> MAELRMEHIYKFYDQKEPAVDDFNLHIADKEFIVFVGPSGCGASTTLRMVAGLEEISKGDFYIEGKRVNDVAPKDRDIAMVFQNYALYPHMTVYDNIAFGLKLRKMPKPEIKKRVEEAAKILGLEEYLHRKPKALSGGQRQRVALGRAIVRDAKVFLMDEPLSNLDAKLRVQMRAEIIKLHQRLQTTTIYVTHDQTEALTMATRIVVMKDGKIQQIGTPKDVYEFPENVFVGGFIGSPAMNFFKGKLTDGLIKIGSAALTVPEGKMKVLREKGYIGKEVIFGIRPEDIHDELIVVESYKNSSIKAKINVAELLGSEIMIYSQIDNQDFIARIDARLDIQSGDELTVAFDMNKGHFFDSETEVRIRLEHHHHHH

ABC exporters and importers share a core structural design composed of at least two intracellular nucleotide-binding domains (NBDs) and two transmembrane domains (TMDs) embedded in the lipid bilayer that form the translocation pore, and the same mechanism of ATP binding and catalysis to energize the movement of substrates across the membrane. Later, our laboratory and others demonstrated that Gram-positive bacteria have orphan NBDs that are able to energize multiple ABC type I sugar importers. Finally, we solve the crystal structure of the B. subtilis multitask ATPase MsmX K43A; the crystals diffracted up to 1.67 Å resolution and based on comparative analysis we hypothesize about sequence and structural features involved in the broader specificity of NBDs. MsmX K43A shares the fold of well-studied NBDs of ABC type I importers.

K43 is involved in ATP coordination and catalysis, interacting with the β- and γ-phosphate groups. Its replacement by an alanine resulted in 80% decreased ATPase activity, impairing the normal function of MsmX to energize the AraNPQ transporter in B. subtilis. The crystal structure was solved at 1.67 Å resolution and the final electron density map allowed to model a detailed refined structure, which comprises all residues of MsmX K43A, except the N-terminus methionine. Interestingly, most crystal structures of NBDs from ABC transporters show a dimer in the asymmetric unit, promoted either by the C-terminal domains or the presence of ATP (or analogs). This is not the case for B. subtilis MsmX, that crystallized as a monomer with one molecule in the asymmetric unit, and very few contacts with symmetry related molecules, as indicated by analyzing the protein interface using PISA server. MsmX N-terminal domain presents the general α/β-type ATPase domain fold, which comprises the RecA-like domain (residues 2–87 and 155–235, in blue) and the α-helical domain (residues 88–154, in yellow). The regulatory C-terminal domain (residues 236–365, in red) forms a mixed barrel with 3 α-helices and 11 β-strands. In the ligand-free MsmX K43A structure here reported, the A-loop length is similar to the one in ATP-bound MalK, already in a conformation that favours nucleotide binding. The MalK F81-Y87 region accommodates the MalF/G helix, providing an hydrophobic environment; in MsmX, the corresponding phenylalanine (F82) is flipped, causing the side chains of Q83 and N84 to point towards the complex interface, which decreases the hydrophobic character of the cleft. Furthermore, in the hydrophobic pocket involved at the interface with the MalF/G, MalK A73 is at 3 Å from the MalF helix, while in MsmX this residue is replaced by K74, which affects considerably the electrostatic potential, the volume and the hydrophobicity of the corresponding pocket.> MYSKIKISGTIEVVTGLHIGGGGESSMIG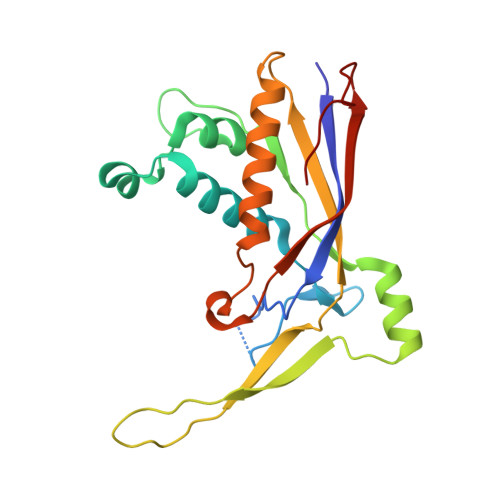AIDSPVVRDLQTKLPIIPGSSIKGKMRNLLAKHFGLKMKQESHNQDDERVLRLFGSSEKGNIQRARLQISDAFFSEKTKEHFAQNDIAYTETKFENTINRLTAVANPRQIERVTRGSEFDFVFIYNVDEESQVEDDFENIEKAIHLLENDYLGGGGTRGNGRIQFKDTNIETVVGEYDSTNLKIK> WQFTPNTGGNTITKVEAENMKIGGTYAG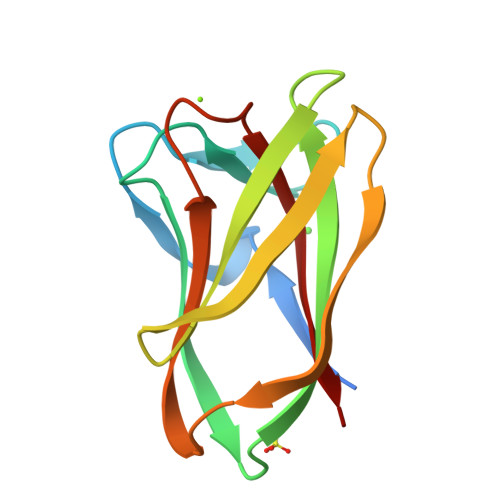KISAPFDGVALYANADYVSYSQYFANSTHNISVRGASSNAGTAKVDLVIGGVTVGSFNFTGKTPTVQTLSNITHATGDQEIKLALTSDDGTWDAYVDFIEFSL>[6x]MASITDKDHQKVILVGDGAVGSSYAYAMVLQGIAQEIGIVDIFKDKTKGDAIDLSNALPFTSPKKIYSAEYSDAKDADLVVITAGAPQKPGETRLDLVNKNLKILKSIVDPIVDSGFNGI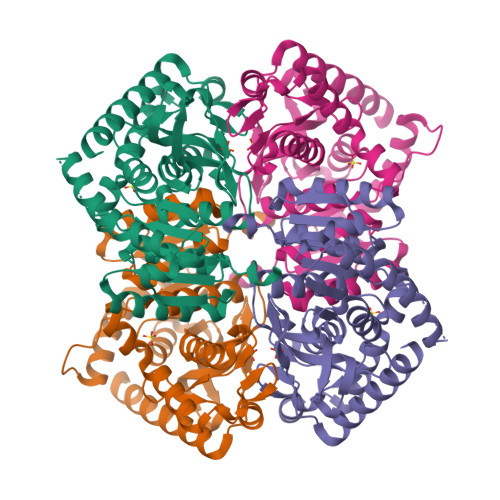FLVAANPVDILTYATWKLSGFPKNRVVGSGTSLDTARFRQSIAEMVNVDARSVHAYIMGEHGDTEFPVWSHANIGGVTIAEWVKAHPEIKEDKLVKMFEDVRDAAYEIIKLKGATFYGIATALARISKAILNDENAVLPLSVYMDGQYGLNDIYIGTPAVINRNGIQNILEIPLTDHEEESMQKSASQLKKVLTDAFAKNDIETRQ>[2x]HHHHHHGSMQILLANPRGFCAGVDRAISIVENALAIYGAPIYVRHEVVHNRYVVDSLRERGAIFIEQISEVPDGAILIFSAHGVSQAVRNEAKSRDLTVFDATCPLVTKVHMEVARAS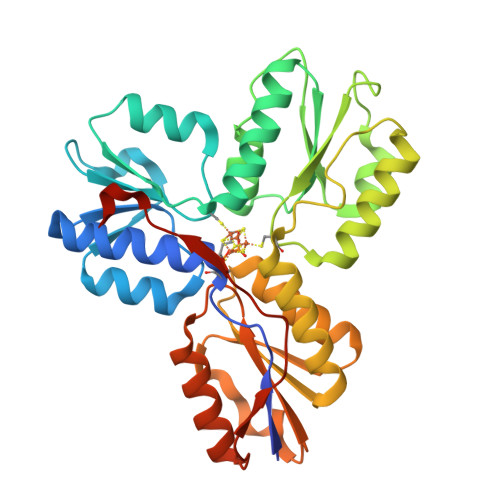RRGEESILIGHAGHPEVEGTMGQYSNPEGGMYLVESPDDVWKLTVKNEEKLSFMTQTTLSVDDTSDVIDALRKRFPKIVGPRKDDICYATTNRQEAVRALAEQAEVVLVVGSKNSSNSNRLAELAQRMGKRAFLIDDAKDIQEEWVKEVKCVGVTAGASAPDILVQNVVARLQQLGGGEAIPLEGREENIVFEVPKELRVDIREVD> KAA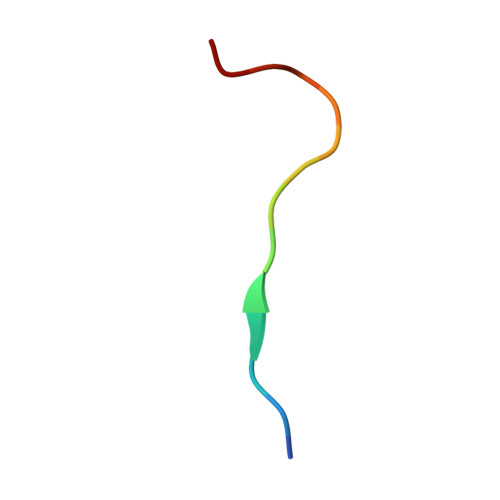RKSAPATGGVK> QGPLGSSKVSEQLKCCSGILKEMFAKKHAAYAWPFYKPVDVEALGLHDY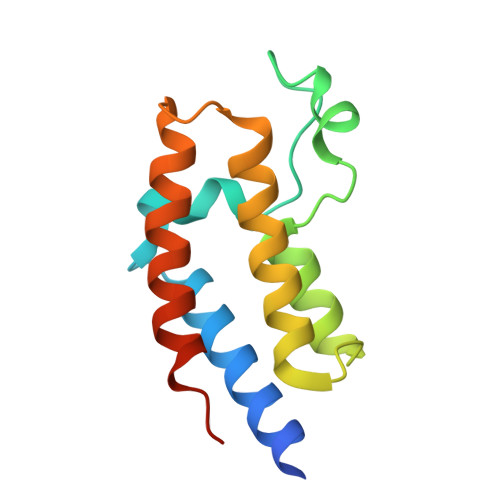CDIIKHPMDMSTIKSKLEAREYRDAQEFGADVRLMFSNCYKYNPPDHEVVAMARKLQDVFEMRFAKMPDEPEEP>MQWQTKLPLIAILRGITPDEALAHVGAV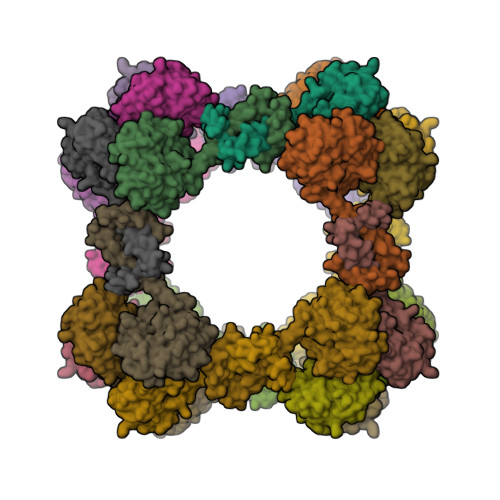IDAGFDAVEIPLNSPQWEQSIPAIVDAYGDKALIGAGTVLKPEQVDALARMGCQLIVTPNIHSEVIRRAVGYGMTVCPGCATATEAFTALEAGAQALKIFPSSAFGPQYIKALKAVLPSDIAVFAVGGVTPENLAQWIDAGCAGAGLGSDLYRAGQSVERTAQQAAAFVKAYREAQKQKEQRQDQKSAYALGASLGRYMENSLKEQEKLGIKLDKDQLIAGVQDAFADKSKLSDQEIEQTLQAFEARVKSSAQAKLEHHHHHH[2x]>MGCWGRNRGRLLCMLALTFMFMVLEVVVSRVTSSLAMLSDSFHMLSNVLALVVALVAERFARRTHATQKNTFGWIRAEVMGALVNAIFLTGLCFAILLEAIERFIEPHEMQQPLVVLGVGVAGLLVNVLGLCLFHHHSGFSQDSGHGHSHGGHGHGHGLPKGPRVKSTRPGSSDINVAPGEQGPDQEETNTLVANTSNSNGLKLDPADPENPRSGDTVEVQVNGNLVREPDHMELEEDRAGQLNMRGVFLHVLGNALGSVIVVVNALVFYFSWKGCSEGDFCVNPCFPDPCKAFVEIINSTHASVYEA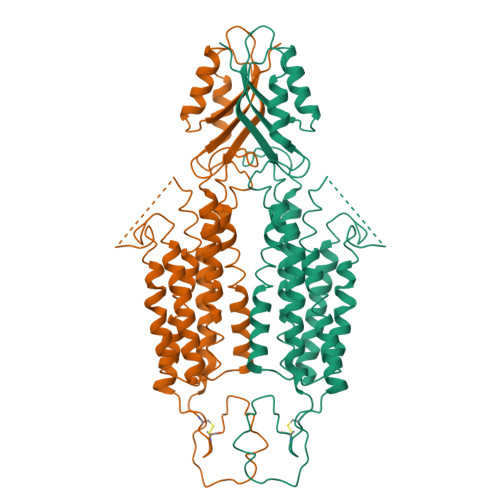GPCWVLYLDPTLCVVMVCILLYTTYPLLKESALILLQTVPKQIDIRNLIKELRNVEGVEEVHELHVWQLAGSRIIATAHIKCEDPTSYMEVAKTIKDVFHNHGIHATTIQPEFASVGSKSSVVPCELACRTQCALKQCCGTLPQAPSGKDAEKTPAVSISCLELSNNLEKKPRRTKAENIPAVVIEIKNMPNKQPESSL[2x]>[2x]GPRNLRVLLDTAIPPSFCDTVSSVLLDDFNMVSLIRTSPADSLATIKQDNAEIDIAITIDEELKISRFNQCVLGYTKAFVVAHPQHPLCNASLHSIASLANYRQISLGSRSGQHSNLL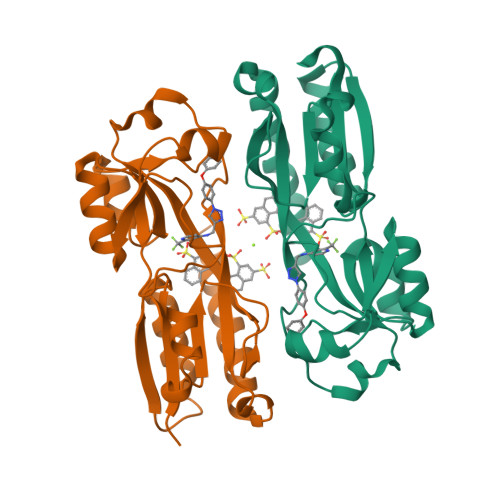RPVSDKVLFVENFDDMLRLVEAGVGWGIAPHYFVEERLRNGTLAVLSELYEPGGIDTKVYCYYNTALESERSFLRFLESARQRLRELGRQRFDDAPAWQPSIVETAQRRSG> QWALEDFEIGRPLGKGKFGNVYLAREKQSKFILALXVLFKAQLEKAGVEHQLRREVEIQSHLRHP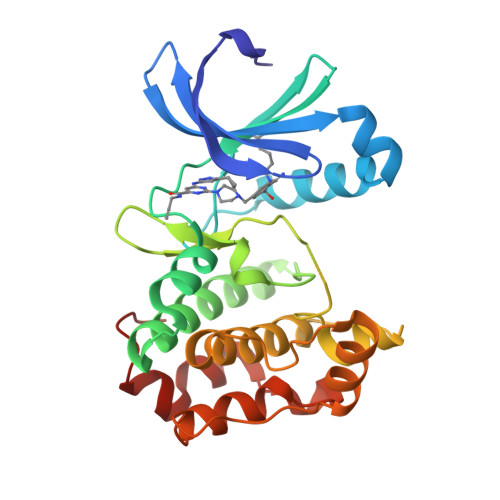NILRLYGYFHDATRVYLILEYAPLGTVYRELQKLSKFDEQRTATYITELANALSYCHSKRVIHRDIKPENLLLGSAGELKIADFGWSVHAPSSRRTTLCGTLDYLPPEMIEGRMHDEKVDLWSLGVLCYEFLVGKPPFEANTYQETYKRISRVEFTFPDFVTEGARDLISRLLKHNPSQRPMLREVLEHPWITANSSKPS> ADPEAFLLFSRRADIRRISLETNNNNVAIPLTGVKEASALDFDVTDNRIYWTDISLKTISRAFMNGSALEHVVEFGLDYPEGMAVDWLG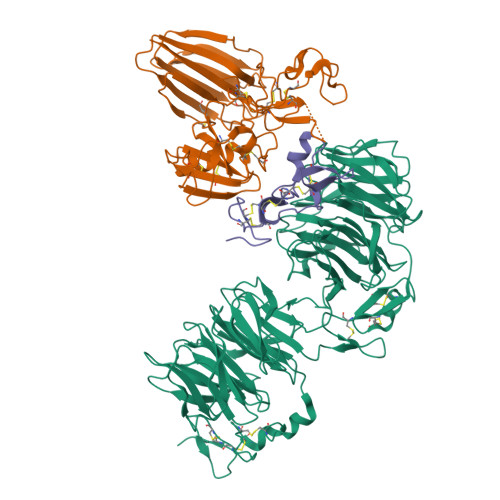KNLYWADTGTNRIEVSKLDGQHRQVLVWKDLDSPRALALDPAEGFMYWTEWGGKPKIDRAAMDGSERTTLVPNVGRANGLTIDYAKRRLYWTDLDTNLIESSNMLGLNREVIADDLPHPFGLTQYQDYIYWTDWSRRSIERANKTSGQNRTIIQGHLDYVMDILVFHSSRQSGWNECASSNGHCSHLCLAVPVGGFVCGCPAHYSLNADNRTCSAPTTFLLFSQKSAINRMVIDEQQSPDIILPIHSLRNVRAIDYDPLDKQLYWIDSRQNMIRKAQEDGSQGFTVVVSSVPSQNLEIQPYDLSIDIYSRYIYWTCEATNVINVTRLDGRSVGVVLKGEQDRPRAIVVNPEKGYMYFTNLQERSPKIERAALDGTEREVLFFSGLSKPIALALDSRLGKLFWADSDLRRIESSDLSGANRIVLEDSNILQPVGLTVFENWLYWIDKQQQMIEKIDMTGREGRTKVQARIAQLSDIHAVKELNLQEYRQHPCAQDNGGCSHICLVKGDGTTRCSCPMHLVLLQDELSCGEP;> PECFTANGADYRGTQNWTALQGGKPCLFWNETFQHPYNTLKYPNGEGGLGEHNYCRNPDGDVSPWCYVAEHEDGVYWKYCEIPACQMPGNLGCYKDHGNPPPLTGTSKTSNKLTIQTCISFCRSQRFKFAGMESGYACFCGNNPDYWKYGEAASTECNSVCFGDHTQPCGGDGRIILFDTLVGACGGNYSAMSSVVYSPDFPDTYATGRVCYWTIRVPGASHIHFSFPLFDIRDSADMVELLDGYTHRVLARFHGRSRPPLSFNVSLDFVILYFFSDRINQAQGFAVLYQAVK;> KGQEGSVCLRSSDCASGLCCARHFWSKICKPVLKEGQVCTKHRRKGSHGLEIFQRCYCGEGLSCRIQKDHHQASNSSRLHTCQRH> XFTGVQGRVIGYDILRSPEVDKAKPLFTETQWDGSELPIYDAKPLQDALVEYFGTEQDRRHYPAPGSFIVCANKGVTAERPKNDADMKPGQGYGVWSAIAISFAKDPTKDSSMFVEDAGVWETPNEDELLEYLEGRRKAMAKSIAECGQDAHASFESSWIGFAYTMMEPGQIGNAITVAPYVSLPIDSIPGGSILTPDKDMEIMENLTMPEWL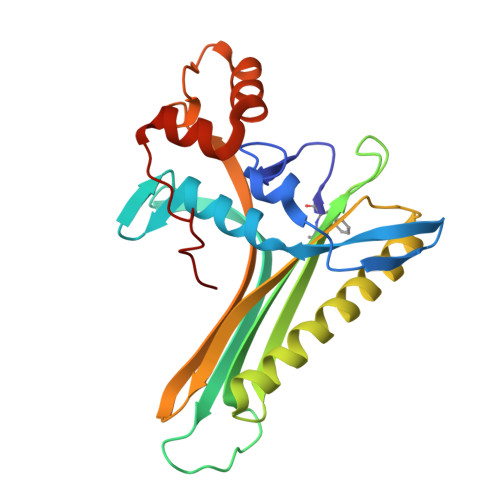EKMGYKSLSANNALKY>MGVVNVPSNGREKFKKNWKFCVGTGRLGLALQKEYLDHLKLVQEKIGFRYIRGHGLLSDDVGIYREVEIDGEMKPFYNFTYIDRIVDSYLALNIRPFIEFGFMPKALASGDQTVFYWKGNVTPPKDYNKWRDLIVAVVSHFIERYGIEEVRTWLFEVWNAPNLVNFWKDANKQEYFKLYEVTARAVKSVDPHLQVGGPAICGGSDEWITDFLHFCAERRVPVDFVSRHAYTSKAPHKKTFEYYYQELEPPEDMLEQFKTVRALIRQSPFPHLPLHITEYNTSYSPINPVHDTALNAAYIARILSEGGDYVDSFSYWTFSDVFEEMDVPKALFHGGFGLVALHSIPKPTFHAFTFFNALGDELLYRDGEMIVTRRKDGSIAAVLWNLVMEKGEGLTKEVQLVIPVSESAVFIKRQIVNEQYGNAWRVWKQMGRPRFPSRQAVETLRQVAQPHVMTEQRRATDGVIHLSI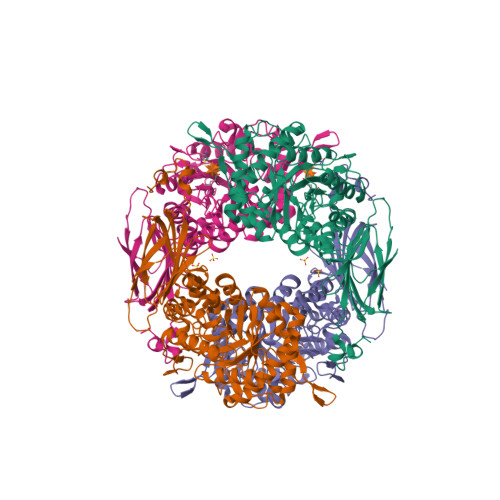VLSKNEVTLIEIEQVRDETSTYVGLDDGEITSYSS[8x]>MGSSHHHHHHSSGLVPRGSHMASATASRGASQAGAPQGRVPEARPNSMVVEHPEFLKAGKEPGLQIWRVEKFDLVPVPTNLYGDFFTGDAYVILKTVQLRNGNLQYDLHYWLGNECSQDESGAAAIFTVQLDDYLNGRAVQHREVQGFESATFLGYFKSGLKYKKGGVASGFKHVVPNEVVVQRLFQVKGRRVVRATEVPVSWESFNNGN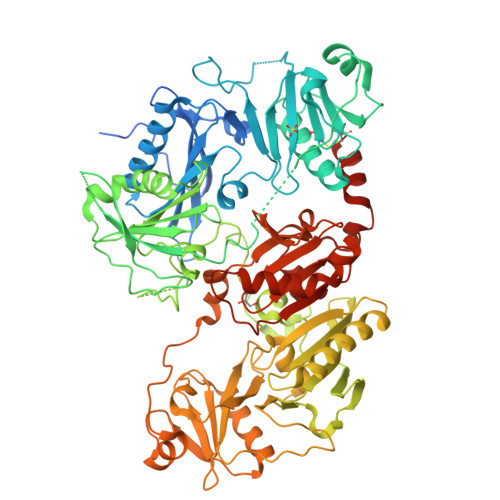CFILDLGNNIHQWCGSNSNRYERLKATQVSKGIRDNERSGRARVHVSEEGTEPEAMLQVLGPKPALPAGTEDTAKEDAANRKLAKLYKVSNGAGTMSVSLVADENPFAQGALKSEDCFILDHGKDGKIFVWKGKQANTEERKAALKTASDFITKMDYPKQTQVSVLPEGGETPLFKQFFKNWRDPDQTDGLGLSYLSSHIANVERVPFDAATLHTSTAMAAQHGMDDDGTGQKQIWRIEGSNKVPVDPATYGQFYGGDSYIILYNYRHGGRQGQIIYNWQGAQSTQDEVAASAILTAQLDEELGGTPVQSRVVQGKEPAHLMSLFGGKPMIIYKGGTSREGGQTAPASTRLFQVRANSAGATRAVEVLPKAGALNSNDAFVLKTPSAAYLWVGTGASEAEKTGAQELLRVLRAQPVQVAEGSEPDGFWEALGGKAAYRTSPRLKDKKMDAHPPRLFACSNKIGRFVIEEVPGELMQEDLATDDVMLLDTWDQVFVWVGKDSQEEEKTEALTSAKRYIETDPANRDRRTPITVVKQGFEPPSFVGWFLGWDDDYWSVDPLDRAMAELAA[2x]> IEALVPAWDSDIIFKCLCYFHTLYPGLIPLETFPPATIFNFKQKIISILEDKKAVLRGEPIKGPLPICCSKENYRRHLQRTTLL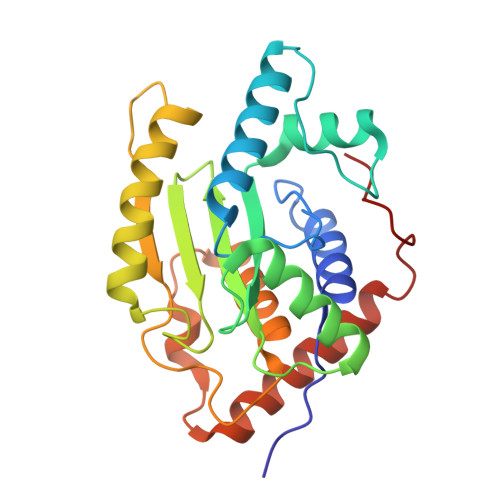PVFMWYHPTPKTLSDTMQTMKQLAIKGSVGASHWLLVIVDIQARRLVYFDSLYNYVMPPENMKKELQSFAQQLDQVYPAYDSKKFSVKIAAKEVIQRGSGSSCGAWCCQFLHWYLKDPLTDALNDLPVDSVERHENLASFVQACEAAVQDLPELSWPEA> GPLGSLTMGAQDTLPVAAAFTETVNAYFKGADPSKCIVKITGEMVLSFPAGITRHFANNPSPAALTFRVINFSRLEHVLPNPQLLCCDNTQNDANTKEFWVNMPNLMTHLKKVSEQKPQATYYNVDMLKYQVSAQGIQSTPLNLAVNWRCEPSSTDLRIDYKYNTDAMTTAVALNNVQFLVPIDGGVTKLQAVLPPAVWNAEQQRILWKIPDISQKSENGGVGSLLARFQLSEGPSKPSPLVVQFTSEGSTLSGCDIELVGAGYRFSLIKKRFAAGKYLADN;> YDPFGGDPFKG

Src homology 3 (SH3)-domain growth factor receptor-bound 2-like (endophilin) interacting protein 1 (SGIP1) and its splicing variant, SGIP1α, are brain-specific homologs of FCHo1/FCHo2. The μHDs of SGIP1 and SGIP1α, which are identical to each other, are highly homologous to those of FCHo1/FCHo2. The μHD of SGIP1/SGIP1α also binds to the DPF motif-rich region of Eps1519. Thus, the SGIP1/FCHo1/FCHo2 μHD is a domain designed for recognizing the locally ordered structure formed by the two consecutive DPF motifs.

We next crystallized the complex between the SGIP1 μHD and two short μHD-binding Eps15 fragments containing two DPF motifs derived from the high-affinity μHD-binding site, Eps15-640–649 and Eps15-645–654. In the two structures, the two DPF motifs are recognized by a continuous cleft on the μHD. The two DPF motifs in the two structures adopt type-I β-turn conformations, and each is stabilized by two sequence-specific intramotif interactions. In our complex structures, the two DPF motifs are intimately packed against each other through hydrophobic interactions between the side chains of Phe in the N-terminal DPF motif and Pro in the C-terminal DPF motif. This arrangement of the DPF motifs brings the hydrophobic side chains of all of the Pro and Phe residues of the two DPF motifs together on one side, allowing their extensive recognition by the continuous hydrophobic cleft of the μHD. Two conserved Ala residues, Ala563 and Ala565, of SGIP1 are located at the bottom of this recognition cleft. Ala563 contacts the side chains of Phe in the N-terminal DPF motif and Pro in the C-terminal DPF motif, while Ala565 contacts the side chains of Pro and Phe in the N-terminal DPF motif. In the two structures, the two DPF motifs bind to the same recognition cleft on the μHD. However, the positions of the C-terminal DPF motif relative to the recognition cleft slightly differ between the two structures, probably due to differences in the lengths and the amino acid sequences of the linker region between the two DPF motifs. Nevertheless, the key interactions for DPF motif recognition by the μHD are essentially conserved in the two structures (see below).>MSPILGYWKIKGLVQPTRLLLEYLEEKYEEHLYERDEGDKWRNKKFELGLEFPNLPYYIDGDVKLTQSMAIIRYIADKHNMLGGCPKERAEISMLEGAVLDIRYGVSRIAYSKDFETLKVDFLSKLPEMLKMFEDRLCHKTYLNGDHVTHPDFMLYDALDVVLYMDPMCLDAFPKLVCFKKRIEAIP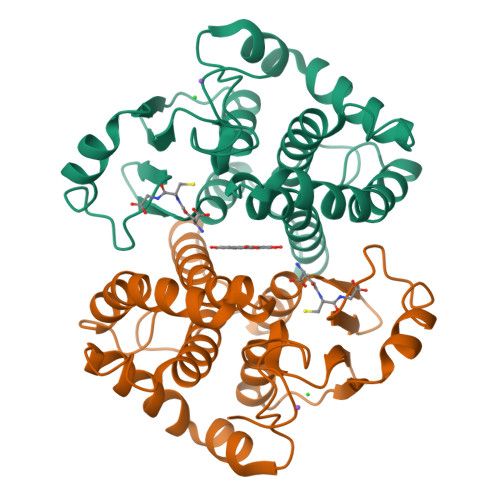QIDKYLKSSKYIAWPLQGWQATFGGGDHPPK[2x]> MVILGVGYFLLGLILLYYGSDWFV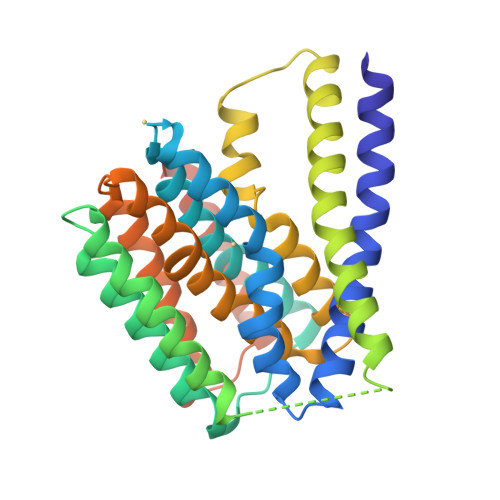LGSERIARHFNVSNFVIGATVMAIGTSLPEILTSAYASYMHAPGISIGNAIGSCICNIGLVLGLSAIISPIIVDKNLQKNILVYLLFVIFAAVIGIDGFSWIDGVVLLILFIIYLRWTVKNGSAEIEENNDKNNPSVVFSLVLLIIGLIGVLVGAELFVDGAKKIALALDISDKVIGFTLVAFGTSLPELMVSLAAAKRNLGGMVLGNVIGSNIADIGGALAVGSLFMHLPAENVQMAVLVIMSLLLYLFAKYSKIGRWQGILFLALYIIAIASLRMGGGSLVPRGSRSHHHHHHH(4M)-4-[1-(2-methoxyethyl)-1H-pyrazol-4-yl]-N-({4-[(propan-2-yl)oxy]phenyl}methyl)quinolin-8-amine 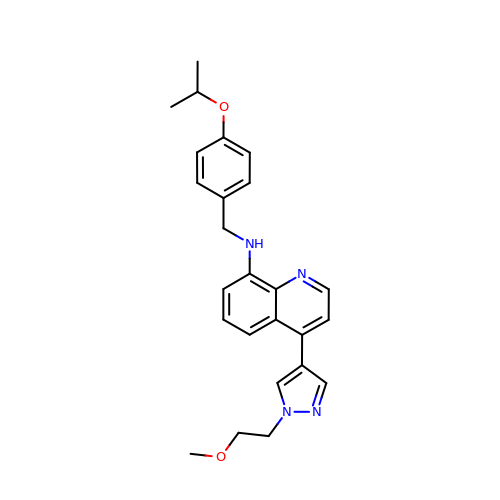| C25 H28 N4 O2 | VNUCWASRIWPIJH-UHFFFAOYSA-N> SGDMAAEVYFGDLELFEPFDHPEESIPKPVHTRFKDDDGDEEDENGVGDAELRERLRQCEETIEQLRAENQELKRKLNILTRPSGILVNDTKLDGPILQILFMNNAISKQYHQEIEEFVSNLVKRFEEQQKNDVEKTSFNLLPQPSSIVLEEDHKVEESCAIKNNKEAFSVVGSVLYFTNFCLDKLGQPLLNENPQLSEGWEIPKYHQVFSHIVSLEGQEIQVKAKRPKPHCFNCGSEEHQMKDCPMPRNAARISEKRKEYMDACGEANNQNFQQRYHAEEVEERFGRFKPGVISEELQDALGVTDKSLPPFIYRMRQLGYPPGWLKEAELENSGLALYDGKDGTDGETEVGEIQQNKSVTYDLSKLVNYPGFNISTPRGIPDEWRIFGSIPMQACQQKDVFANYLTSNFQAPGVKSGGAVDEDALTLEELEEQQRRIWAALEQAESVNSDSDVPVDTPLTGNSVASSPCPNELDLPVPEGKTSEKQTL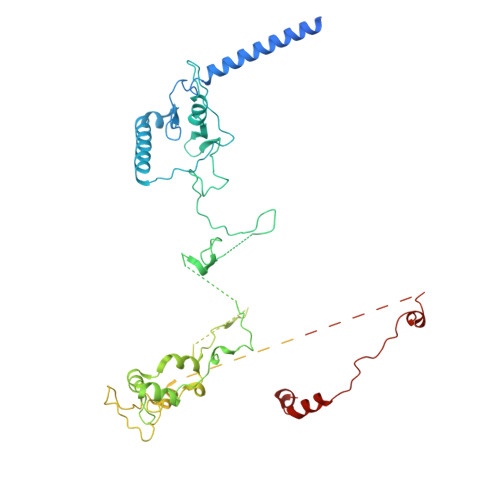DEPEVPEIFTKKSEAGHASSPDSEVTSLCQKEKAELAPVNTEGALLDNGSVVPNCDISNGGSQKLFPADTSPSTATKIHSPIPDMSKFATGITPFEFENMAESTGMYLRIRSLLKNSPRNQQKNKKASE>[4x]ALGSVTDRHAAEYNMRHKNRGMALIFNHEHFEVPTLKSRAGTNVDCENLTRVLKQLDFEVTVYKDCRYKDILRTIEYS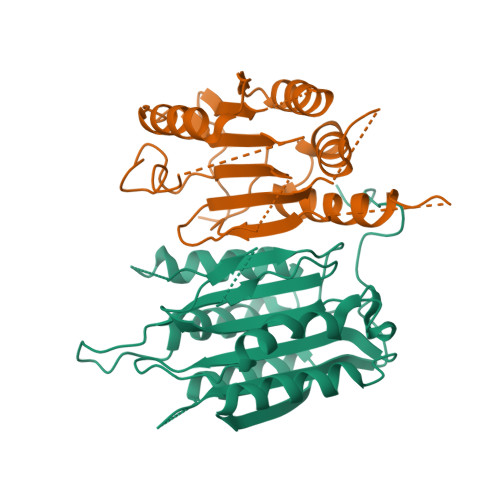ASQNHSDSDCILVAILSHGEMGYIYAKDTQYKLDNIWSFFTANHCPSLAGKPKLFFIQACQGDRLDGGVTMQRSQTETDGDSSMSYKIPVHADFLIAYSTVPGFYSWRNTTRGSWFMQSLCAELAANGKRLDILTLLTFVCQRVAVDFESCTPDTPEMHQQKQIPCITTMLTRILRFSDKQ>MLKDGDYTVETAKADDHGYKAKLSIKVSDGKITEAKYNEFNGETNAMKREDKDYNEKMTGVSGIGPAEYEPQLEKALIEKQSSDIDVITGATSSSNQFKKLA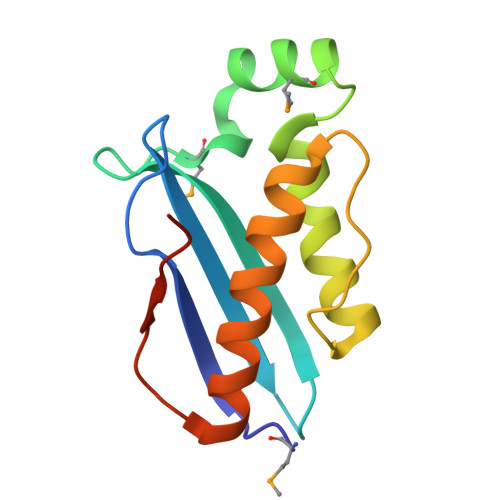EKVLKNAEEGKTEATLVDLEHHHHHH[5x]>[3x]MGAVAVDLGNRKLEISSGKLARFADGSAVVQSGDTAVMVTAVSKTKPSPSQFMPLVVDYRQKAAAAGRIPTNYLRREVGTSDKEILTSRIIDRSIRPLFPAGYFYDTQVLCNLLAVDGVNEPDVLAINGASVALSLSDIPWNGPVGAVRIGIIDGEYVVNPTRKEMSSSTLNLVVAGAPKSQIVMLEASAENILQQDFCHAIKVGVKYTQQIIQGIQQLVKETGVTKRTPQKLFTPSPEIVKYTHKLAMERLYAVFTDYEHD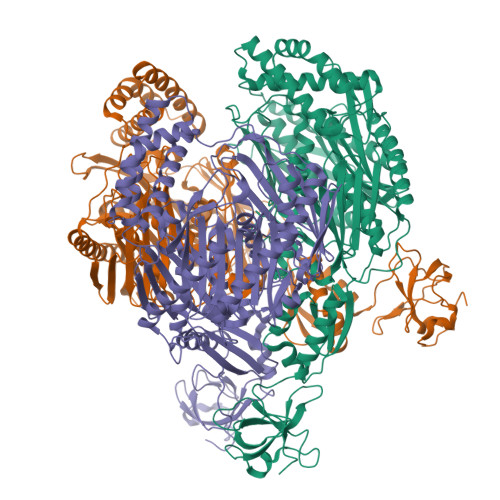KVSRDEAVNKIRLDTEEQLKEKFPEADPYEIIESFNVVAKEVFRSIVLNEYKRCDGRDLTSLRNVSCEVDMFKTLHGSALFQRGQTQVLCTVTFDSLESGIKSDQVITAINGIKDKNFMLHYEFPPYATNEIGKVTGLNRRELGHGALAEKALYPVIPRDFPFTIRVTSEVLESNGSSSMASACGGSLALMDSGVPISSAVAGVAIGLVTKTDPEKGEIEDYRLLTDILGIEDYNGDMDFKIAGTNKGITALQADIKLPGIPIKIVMEAIQQASVAKKEILQIMNKTISKPRASRKENGPVVETVQVPLSKRAKFVGPGGYNLKKLQAETGVTISQVDEETFSVFAPTPSAMHEARDFITEICKDDQEQQLEFGAVYTATITEIRDTGVMVKLYPNMTAVLLHNTQLDQRKIKHPTALGLEVGQEIQVKYFGRDPADGRMRLSRKVLQ> MGHHHHHHHHHHSSG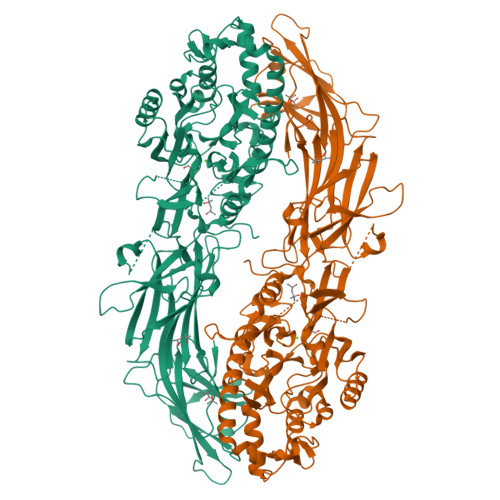HIEGRHMLRERTVRLQYGSRVEAVYVLGTYLWTDVYSAAPAGAQTFSLKHSEHVWVEVVRDGEAEEVATNGKQRWLLSPSTTLRVTMSQASTEASSDKVTVNYYDEEGSIPIDQAGLFLTAIEISLDVDADRDGVVEKNNPKKASWTWGPEGQGAILLVNCDRETPWLPKEDCRDEKVYSKEDLKDMSQMILRTKGPDRLPAGYEIVLYISMSDSDKVGVFYVENPFFGQRYIHILGRRKLYHVVKYTGGSAELLFFVEGLCFPDEGFSGLVSIHVSLLEYMAQDIPLTPIFTDTVIFRIAPWIMTPNILPPVSVFVCCMKDNYLFLKEVKNLVEKTNCELKVCFQYLNRGDRWIADEIEFGYIEAPHKGFPVVLDSPRDGNLKDFPVKELLGPDFGYVTREPLFESVTSLDSFGNLEVSPPVTVNGKTYPLGRILIGSSFPLSGGRRMTKVVRDFLKAQQVQAPVELYSDWLTVGHVDEFMSFVPIPGTKKFLLLMASTSACYKLFREKQKDGHGEAIMFKGLGGMSSKRITINKILSNESLVQENLYFQRCLDWNRDILKKELGLTEQDIIDLPALFKMDEDHRARAFFPNMVNMIVLDKDLGIPKPFGPQVEEECCLEMHVRGLLEPLGLECTFIDDISAYHKFLGEVHCGTNVRRKPFTFKWWHMVPSRRS> GSGPIDFWSSHPGQSSAAERELIGRFQDRFPTLSVKLIDAGKDYDEVAQKFNAALIGTDVPDVVLLDDRWWFHFALSGVLTALDDLFGQVGVDTTDYVDSLLADYEFNGRHYAVPYARSTPLFYYNKAAWQQAGLPDRGPQSWSEFDEWGPELQRVVGAGRSAHGWANADLIS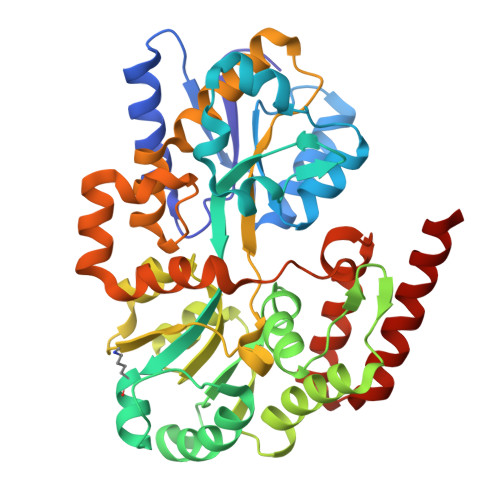WTFQGPNWAFGGAYSDKWTLTLTEPATIAAGNFYRNSIHGKGYAAVANDIANEFATGILASAVASTGSLAGITASARFDFGAAPLPTGPDAAPACPTGGAGLAIPAKLSEERKVNALKFIAFVTNPTNTAYFSQQTGYLPVRKSAVDDASERHYLADNPRARVALDQLPHTRTQDYARVFLPGGDRIISAGLESIGLRGADVTKTFTNIQKRLQVILDRQIM5-chloro-1H-benzimidazole | C7 H5 Cl N2 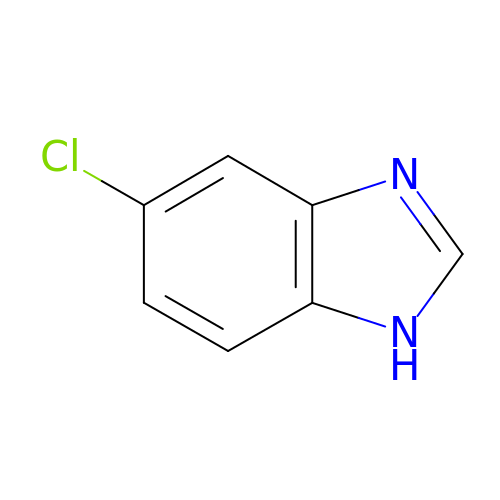| NKLOLMQJDLMZRE-UHFFFAOYSA-N Argonaute proteins are programmable nucleases that have defense and regulatory functions in both eukaryotes and prokaryotes. Here, we describe a new class of pAgos that uniquely use DNA guides to process RNA targets. The biochemical and structural analysis of Pseudooceanicola lipolyticus pAgo (PliAgo) reveals an unusual organization of the guide binding pocket that does not rely on divalent cations and the canonical set of contacts for 5’-end interactions. Unconventional interactions of PliAgo with the 5’-phosphate of guide DNA define its new position within pAgo and shift the site of target RNA cleavage in comparison with known Argonautes.

To elucidate the mechanism of guide DNA binding and cleavage site selection by the newly identified D-R pAgos, we determined 3D structures of apo-form PliAgo and of its complex with 5’-phosphorylated guide DNA (P-gDNA, 18 nt long), either in the absence or in the presence of Mg2+. The structure of PliAgo was determined by single wavelength anomalous dispersion (SAD) method with SeMet labeled protein at 3.28 Å resolution followed by extending the final resolution to 3.1 Å with a native crystal. All crystals were formed at nearly identical crystallization conditions and belonged to the same space group, containing one PliAgo or PliAgo-DNA complex per asymmetric unit. A crescent-shaped PliAgo molecule contains the N-terminal-L1-PAZ domains on one side and the L2-MID-PIWI domains on the other side, similar to other eAgos and pAgos such as TtAgo. In contrast, the C-terminal 18–20 residues of PliAgo are disordered in all the structures indicating that the C-terminus is located away from the 5’-end binding pocket and does not interact with guide DNA.

> MTLETTLFPLEGLEGLTASYQLYAVKGLSGLDETEYHKNVNLLVRRLSFSMKAPFVALSRDGEQFIAVPNYVTEFPVDHRVVRAMVKLVPTGEPLNLRFDAADDEYDGLRLRYLDFVLQQPLFANHHLWQPGSGQPFFHKKPLKRLDDVDLYDGVSVRAAKHPEGGFGIVCDARSKFITHTPIGARADRKRLGKLINRSCLYKMGDHWYQFRIDAVSDWKVGEPSLFEGNVPISLAQQLVRTAGNAAPKSIIDLDPEGGALEYFTSTNERRMAPAELCFLIEDTHGRRAAKLQRQTILSPSERRARVNGFIRRYLSELNIGGAKLSAGARAHAFFTETHMPPALSFGNGTVLAPDTSKDRFQAMQEYSSMRRTMMLDKKVGFFHQDVFPPQTLLLPESVKKSWGPAFASDFVGTVQELYPAGGYRPEIIEYRDKAYGGGVPGQMKALLEVAERGEIKSGDVLVMLHRINGAPRAQDKLAAMVCNEFEKRFGKRVQVIHSDSPGRGYKRIFKNDKPTYVQQRGRGVNIKGYLKGAALNKVCLGNSRWPFVLRDPLNADVTIGIDVKNNMAVFTMVAEGGRIVRVQRSRSRQREQLLESQVTQVITEMLSKELPEIKKQVQRVVIHRDGRAWPAEIAGARKTFADMAESGLIAVDADVSVFEVLKSSPAPLRLFSFEEPTQENPKGVINPVLGSWLKLSENDGYICTTGAPLLLQGTADPLHVRKAFGPMAIEDALKDVFDLSCLTWPKPDSCMRLPLTIKLCDIALFDDAAEYDVDVVRFADGNTGEASA>[2x]SNAMKVKIYTRNGCPYCVWAKQWFEENNIA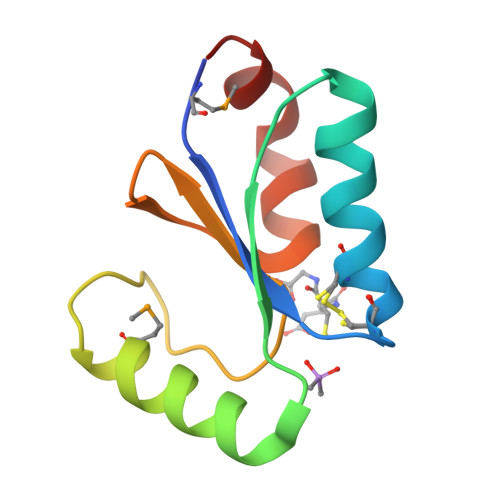FDETIIDDYAQRSKFYDEMNQSGKVIFPISTVPQIFIDDEHIGGFTELKANADKILNKK> DVFQNKANVCWAKA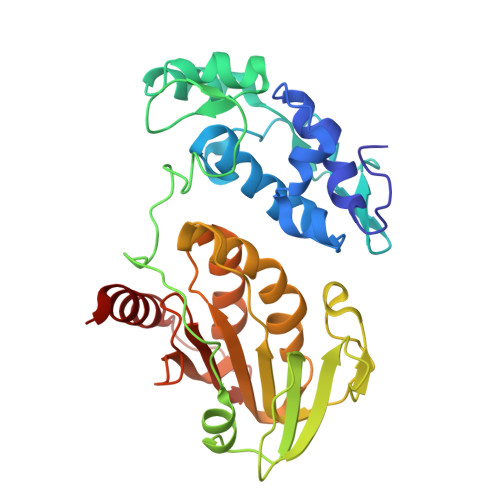LVPVLKTAGIDMTTEQWNTVDYFETDKAHSAEIVLNQLCVRFFGLDLDSGLFSAPTVPLSIRNNHWDNSPSPNMYGLNKEVVRQLSRRYPQLPRAVATGRVYDMNTGTLRNYDPRINLVPVNRRLPHALVLHHNEHPQSDFSSFVSKLKGRTVLVVGEKLSVPGKMVDWLSDRPEATFRARLDLGIPGDVPKYDIIFVNVRTPYKYHHYQQCEDHAIKLSMLTKKACLHLNPGGTCVSIGYGYADRASESIIGAIARQFKFSRVCKPKSSLEETEVLFVFIGYDRKARTHNPYKLSSTLTNIYTGS> KEQRLKEQLGAQQEPVKKSIQESEAFLPQSIPEERYKMKSKPLGICLIIDCIGNETELLRDTFTSLGYEVQKFLHLSMHGISQILGQFACMPEHRDYDSF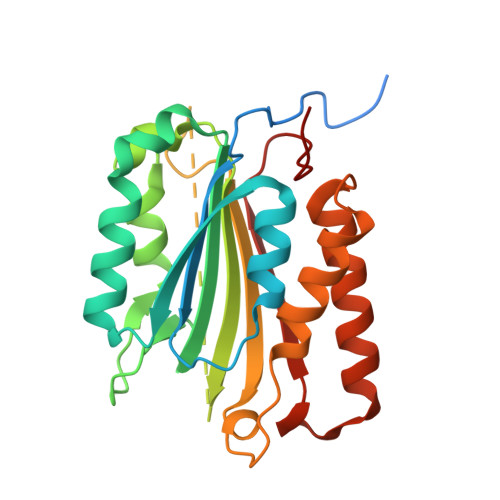VCVLVSRGGSQSVYGVDQTHSGLPLHHIRRMFMGDSCPYLAGKPKMFFIQNYVVSEGQLENSSLLEVDGPAMKNVEFKAQKRGLCTVHREADFFWSLCTADMSLLEQSHSSPSLYLQCLSQKLRQERKRPLLDLHIELNGYMYDWNSRVSAKEKYYVWLQHTLRKKLILSYT>[2x]MKFDPQKYRELAEKDFEAAWKAGKEILAERSPNELYPRVGFSFGKEHPLFATIQRLREAYLSIGFSEVVNPLIVEDVHVKKQFGREALAVLDRCFYLATLPKPNVGISAEKIRQIEAITKREVDSKPLQEIFHRYKKGEIDGDDLSYLIAEVLDVDDITAVKILDEVFPEFKELKPISSTLTLRSHMTTGWFITLSHIADKLPLPIKLFSIDRCFRREQGEDATRLYTYFSASCVLVDEEL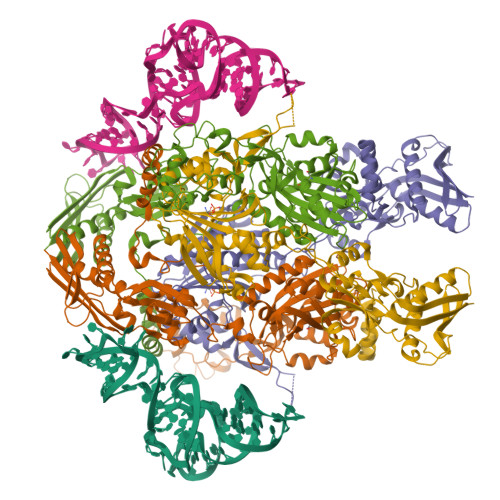SVDDGKAVAEALLRQFGFENFRFRKDEKRSKYYIPDTQTEVFAFHPKLVGSSTKYSDGWIEIATFGIYSPTALAEYDIPYPVMNLGLGVERLAMILYGYDDVRKMVYPQIHGEIKLSDLDIAREIKVKEVPQTAVGLKIAQSIVETAEKHASEPSPCSFLAFEGEMMGRNVRVYVVEEEENTKLCGPAYANEVVVYKGDIYGIPKTKKWRSFFEEGVPTGIRYIDGFAYYAARKVEEAAMREQEEVKVKARIVENLSDINLYIHENVRRYILWKKGKIDVRGPLFVTVKAEIE> MIVKEDSVEAVGAQLKVYHQQYQDKSREYDQLYEEYTRTSQELQMKRTAIEAFNETI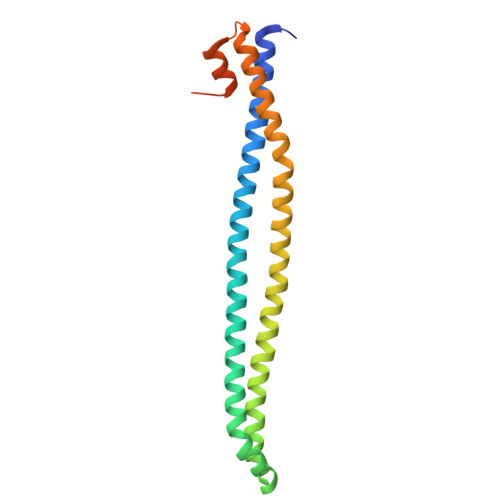KIFEEQGQTQEKCSKEYLERFRREGNEKEMQRILLNSERLKSRIAEIHESRTKLEQQLRAQASDNREIDKRMNSLKPDLMQLRKIRDQYLVWLTQKGARQKKINEWLGIKNETEDQYALMEDLEHHHHHH>SKPFTLPILTLGELTNS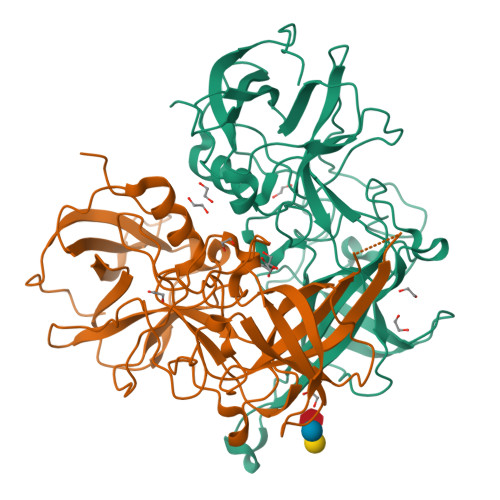RFPLPIDVLYTNPNESAIVQCQNGRCTLDGELQGTTQLLPTGICAFRGKVTQQVQDEHRGTHWNMTVTNLNGTPFDPTEDVPAPLGTPDFSGQIYGVISQRNTNTVPGEGNLPANRAHEAVIATYSPKFTPKLGNIQFSTWETQDVSSGQPTKFTPVGLASVDANSHFDQWTLPSYSGALTLNMNLAPSVAPVFPGECLLFFRSFIPLKGGYGNPAIDCLMPQEWVQHLYQESAPSLSDVALVRYVNPETGRTLFEAKLHRNGFLTVARNSAGPVVAPTNGYFRFDSWVNQFYTLAPM[2x]CAs are a superfamily of ubiquitous zinc metalloenzymes, present in all kingdoms of life, and encoded by at least eight distinct, evolutionarily unrelated gene families (designated α, β, γ, δ, ζ, η, θ and ι) converging in the same crucial reaction, the reverse hydration of CO2 to H+ and HCO3−15–18. CAs were shown to be essential for the worms to establish a robust infection in experimental animals and findings strongly suggests that chemical inhibition of CA from S. mansoni (SmCA) debilitate the worms and curtail the infection. Here, we report on the development of SmCA inhibitors conjugated to the PZQ scaffold as a possible novel therapeutic target for schistosomiasis. All compounds were evaluated for their inhibition profiles on both humans and Schistosoma CAs, X-ray crystal data of SmCA and hCA II in adduct with some inhibitors were obtained allowing the understanding of the main structural factors responsible of activity.

For structural studies, we sought to complement ligand 35c with SmCA and hCA II in order to observe possible differences in the active site interactions. Initially, we solved the crystal structure of SmCA in the presence of 35c at a resolution of 1.79 Å observing a strong density inside the active site fully compatible with the inhibitor. The binding mode of 35c was the classical of this moiety anchoring the sulphonamide group through the catalytic zinc and displacing the water molecule. In addition, compound 35c formed the characteristic hydrogen bond with residue Thr231, stabilising the interaction. Several hydrophobic interactions are observed for both aromatic ring with side chains Val144 and Leu230 and the terminal portion of inhibitor with Ile114 and Pro154. From a superposition of the two complexes, we found no substantial differences occurring between the two complexes of SmCA and hCA II explaining the similar potency of action against the two different CAs. In addition, crystallographic analysis of the schistosome tegumental enzyme SmCA and human CA II complexed with a selection of these inhibitors showed the hydrophobic tails of the inhibitors is located in the both isoforms in the same hydrophobic task, explaining the lack of selectivity.

>[2x]MTYQWLIGIQISLLFVNCICNGSEWSYTNILTGPETWHEHYKNMCSGYYQSPIDLKTDISTLDLKLKTVIIYRNTSSTETTTIQNNGHSAEVKFPRNTWFISFDGILDYKYEIIQMHFHWGNTDDRGSEHTIDGFRFPLEGHIVSFRRQMYSSPSEAIGRPGGLAVLGIMHQIVESIKYEQTAFKAYNNFSGVLNSQFVPPNNSTIDDINLALLLSLLNPSRYFRYLGSLTTPPCTENVLWTVFIDPVLITREQINLFRNLPYGSNEKQTRMGDNFRPIQLLNPIDTLASRTLYRATARSLSLLSLSGILYIMITSQLSVIFL6-[(6-azanyl-4-oxidanyl-naphthalen-2-yl)sulfonylamino]-4-oxidanyl-naphthalene-2-sulfonic acid | C20 H16 N2 O7 S2 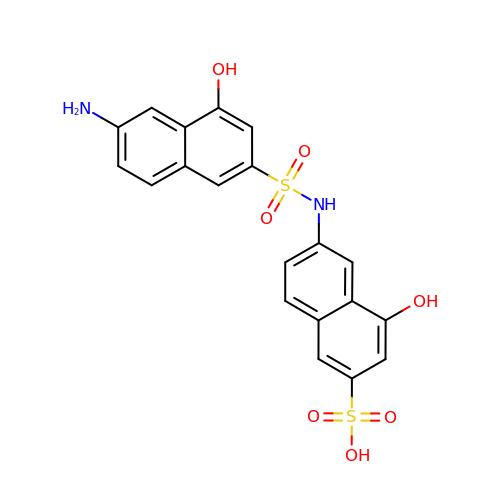| GCIKNRHROSMLPR-UHFFFAOYSA-N3-((R)-4-((3R,5R,8R,9S,10S,13R,14S,17R)-3-(2-hydroxy-2-methylpropyl)-10,13-dimethylhexadecahydro-1H-cyclopenta[a]phenanthren-17-yl)pentanamido)propanoic acid | 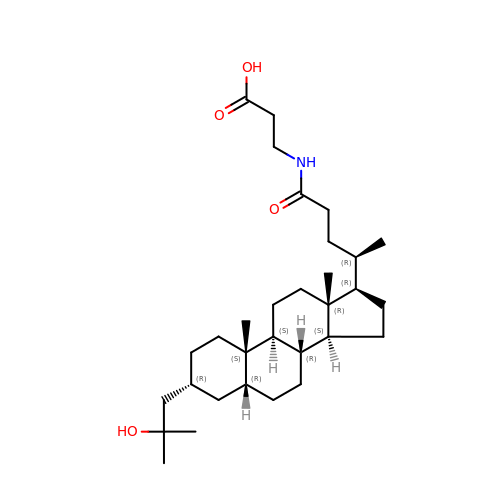C31 H53 N O4 | ZDSAGRUYIZLIJR-XARXUAFMSA-N> SEFFWDVQKIQEISNVEEHSVVKCVTVNTSRLISQLNEELQDEESGVNFIVTQLQLLINNVYEKIQKSPGVPAHRSLMINLNFTRLKFSIAYWDIL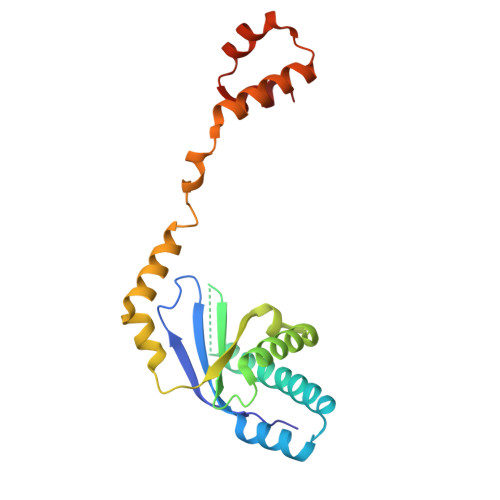LERSLDLINGPSKTGARYFITEVTPVDRSRYVENNQYFLAFKANQRLTRNSVDMDEFIDFEILIKQIIFDLFKKNGIPDQDFEAILSRFHNLESLVVAFNE> MQEKYNFGKVSSQHKNYSKIETMLRPKGFDKLDHYFRTELDIDLTDETIELLLNSVKAAFGKLFYG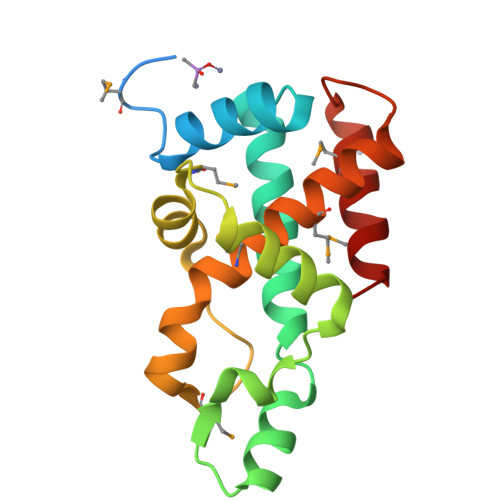AEQRARWNGRDFIALADLNITKALEEHIKNFQKIEQDMGVDELLEYIAFIPPVEMNVGEDLKSEYRNIMGGLLLMHADVIKKATGERKPSREAMEFVAQIVDKVF> QGEFMEPRAVADALETGEEDAVTEALRSFNREHSQSFTFDDAQQEDRKRLAKLLVSVLEQGLSPKHRVTWLQTIRILSRDRSCLDSFASRQSLHALACYADIAISEEPIPQPPDMDVLLESLKCLCNLVLSSPTAQMLAAEARLVVRLAERVGLYRKRSYPHEVQFFDLRLLFLLTALRTDVRQQLFQELHGVRLLTDALELTLGVAPKENPLVILPAQETERAMEILKVLFNITFDSVKREVDEEDAALYRYLGTLLRHCVMADAAGDRTEEFHGHTVNLLGNLPLKCLDVLLALELHEGSLEFMGVNMDVINALLAFLEKRLHQTHRLKECVAPVLSVLTECARMHRPARKFLKAQVLPPLRDVRTRPEVGDLLRNKLVRLMTHLDTDVKRVAAEFLFVLCSESVPRFIKYTGYGNAAGLLAARGLMAGGRPEGQYSEDEDTDTEEYREAKASXXXXXXXXXXXXX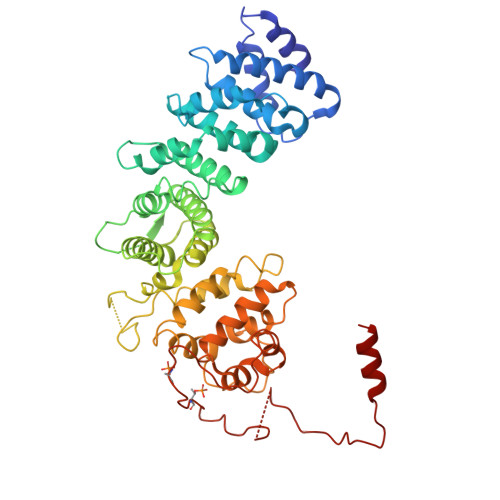XXXXXXXXXXXXXX>MASENNGSRSDSESITAPKADSTVVEPRKIALITGITGQDGSYLTEFLLGKGYEVHGLIRRSSNFNTQRINHIYIDPHNVNKALMKLHYADLTDASSLRRWIDVIKPDEVYNLAAQSHVAVSFEIPDYTADVVATGALRLLEAVRSHTIDSGRTVKYYQAGSSEMFGSTPPPQSETTPFHPRSPYAASKCAAHWYTVNYREAYGLFACNGILFNHESPRRGENFVTRKITRALGRIKVGLQTKLFLGNLQASRDWGFAGDYVEAMWLMLQQEKPDDYVVATEEGHTVEEFLDVSFGYLGLNWKDYVEIDQRYFRPAEVDN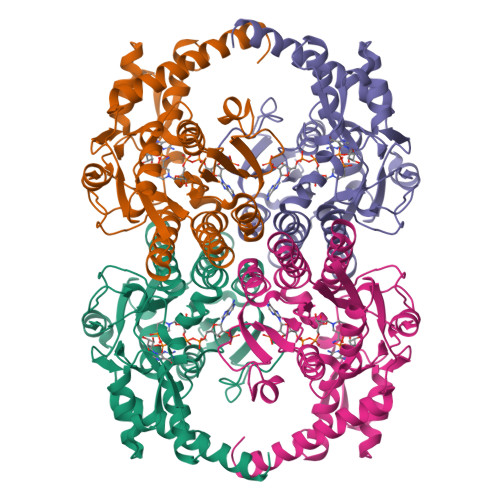LQGDASKAKEVLGWKPQVGFEKLVKMMVDEDLELAKREKVLVDAGYMDAKQQPLEHHHHHH[2x]>SNMATSKVVFITGATSGFGEAAAQVFADAGWSLVLSGRRFERLKTLQDKLASQVPVHIIELDVRDSDSVAAAVAALPADFA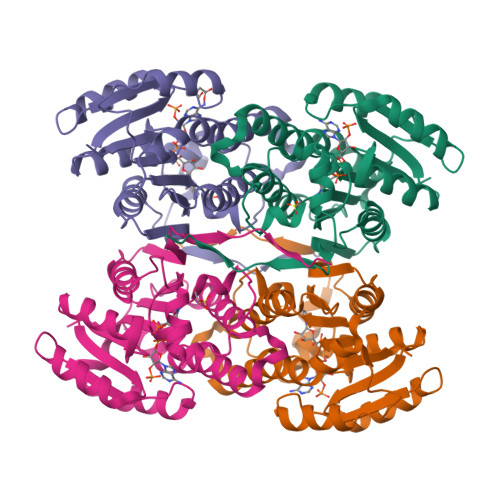DITTLINNAGLALSPQPAQKVDLDDWKTMIDTNVTGLVNVTHALLPTLINHGAGASIINIGSIAGQWPYPGSHVYGASKAFVKQFSYNLRCDLLGTGVRVTDLAPGIAETEFTLVRTKGDQAASDNLYRGTTPLSARDIAEQMFYIATLPDHMNINRVEVMPVRQAWQPFAIDRD[12x]> SIADYKDDDDKMRAEGLGGLERFCSPGKGRGLRALQPFQVGDLLFSCPAYAYVLTVNERGNHCEYCFTRKEGLSKCGRCKQAFYCNVECQKEDWPMHKLECSPMVVFGENWNPSETVRLTARILAKQKIHPERTPSEKLLAVKEFESHLDKLDNEKKDLIQSDIAALHHFYSKHLGFPDNDSLVVLFAQVNCNGFTIEDEELSHLGSAIFPDVALMNHSCCPNVIVTYKGTLAEVRAVQEIKPGEEVFTSYIDLLYPTEDRNDRLRDSYFFTCECQECTTKDKDKAKVEIRKLSDPPKAEAIRDMVRYARNVIEEFRRAKHYKSPSELLEICELSQEKMSSVFEDSNVYMLHMMYQAMGVCLYMQDWEGALQYGQKIIKPYSKHYPLYSLNVASMWLKLGRLYMGLEHKAAGEKALKKAIAIMEVAHGKDHPYISEIKQEIESH

Within the protein lysine methyltransferase (PKMT) family of enzymes, one branch contains five enzymes that share two highly conserved, functional domains: the catalytic SET domain and the MYND domain; these five enzymes are known as SMYD1, SMYD2, SMYD3, SMYD4 and SMYD5. Among the SMYD enzymes, SMYD2 and SMYD3 have been implicated as targets for a variety of cancer indications. In the current study we exemplify pharmacophore series for SMYD2 and SMYD3 that show low nanomolar potency against their targets and significant selectivity over all other enzymes tested with favorable physicochemical properties and pharmacological tractability. S2 Table Crystallographic data collection and refinement statistics for SMYD2 and SMYD3 crystal structures.

EPZ033294 is an inhibitor of SMYD2 that was optimized from an initial hit from Epizyme’s proprietary histone methyltransferase-biased library using a radiometric assay with tritiated SAM and an H3 peptide as substrates. EPZ033294 inhibits the enzymatic activity of SMYD2 with a potency of 3.9 nM and is noncompetitive with respect to peptide substrate and either noncompetitive or uncompetitive with respect to SAM. Instead, SAM dependence was tested by measuring IC50 values at two SAM concentrations differing by 10-fold; the resulting IC50 values were similar, inconsistent with a competitive mechanism. The binding mode suggested by enzyme kinetics is consistent with the crystal structure of the ternary SAM-SMYD2- EPZ033294 complex. The cyclopropyl triazole moiety occupies the lysine channel with the amide carboxyl group hydrogen-bonding to the backbone amide NH of Thr185 and the azetidine nitrogen interacting with the side chain of Glu187; both amino acids are also engaged in hydrogen bonding interactions with peptide substrates. Compared to all other published SMYD2 inhibitors, EPZ033294 binds in a distinct and unique manner, traversing the peptide binding site and inducing a pocket into which the hydrophobic tail of the molecule is inserted. (A) Two molecules of EPZ033294 (molecule 1 = cyan; molecule 2 = purple) were seen in the peptide binding site of SMYD2 (green). SAM (yellow) is show in stick representation. The dissociation constant (KD) was determined to be 5 nM, with a kon = 5 x 105 M-1s-1 and koff = 0.003 s-1. Western blot analysis of intracellular levels of BTF3me1 as a function of EPZ033294 concentration demonstrated a concentration-dependent inhibition of this mark with an IC50 of 2.9 nM.(9aR)-9a-(dioxidanyl)-1,9-dihydrocarbazole | C12 H11 N O2 | 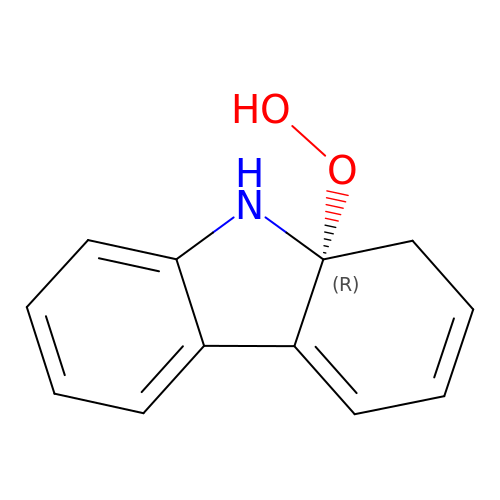UZUUDVVIIUNBSP-GFCCVEGCSA-N N,N'-[acridine-3,6-diylbis(1H-1,2,3-triazole-1,4-diylbenzene-3,1-diyl)]bis[3-(diethylamino)propanamide] 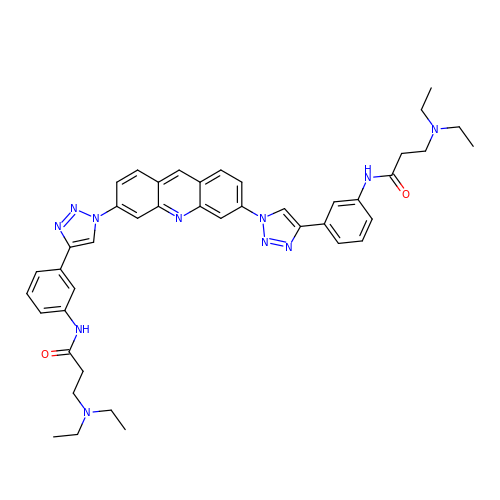| C43 H47 N11 O2 | HZKPUBMHIBOFRM-UHFFFAOYSA-N> MLTRIHGGRVVDPTAGRDAVGDVWIEDGRVVAPSERAPDQTIDATGCVVMAGGVEVHSHIAGGNVVMSRLLLPDLYVSESAPNGHPFAHAGGSGSWIGANYARMGYTTAVEPALPPSNALATHLELADIPLLDRGGLAVLGNDDHLLQLLRDGEGKQAVRDLVQQTLAHSRGLGVKCINAGGASAFKDGVLKLSLDDEIPCYGLSTRKIMSALLDAVEEIGVPHPLHVHCNNLGLPGADDSLVATLEAAEGRRIHFAHAQFYAYGVVDPENPMTGGFRSAAERINAAM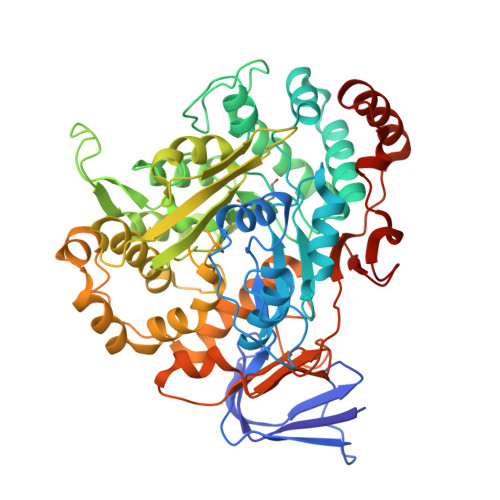EAHPNATYDVGQVVFGQTVTISLDILRQFGGRKGAKPKKWVISAGDAEGGGVVPFLYRPRGPVSSLQWAIGLELMLLSSNPERTILTTDHPNGGVFTEYPRIIHLLMDAEERAKEIATLPAIVGERSGLPKIEREYSFSEIAQLTRSGPAKLLGLTDRGHLREGAKADVAIYRDDTDRTAMFSRAKLVLKDGQPIVEDGEVVAWFSGKTLSLNVEADAGMEKRAESYLQDRFGAGLDTFAVPDAAFPENTGTFEDVACRA> TFISRFAPDQPRKGADILVEALERQGVETVFAYPGGASMEIHQALTRSSSIRNVLPRHEQGGVFAAEGYARSSGKPGICIATSGPGATNLVSGLADALLDSVPLVAITGQVPRRMIGTDAFQETPIVEVTRSITKHNYLVMDVEDIPRIIEEAFFLATSGRPGPVLVDVPKDIQQQLAIPNWEQAMRLPGYMSRMPKPPEDSHLEQIVRLISESKKPVLYVGGGCLNSSDELGRFVELTGIPVASTLMGLGSYPCDDELSLHMLGMHGTVYANYAVEHSDLLLAFGVRFDDRVTGKLEAFASRAKIVHIDIDSAEIGKNKTPHVSVCGDVKLALQGMNKVLENRAEELKLDFGVWRNELNVQKQKFPLSFKTFGEAIPPQYAIKVLDELTDGKAIISTGVGQHQMWAAQFYNYKKPRQWLSSGGLGAMGFGLPAAIGASVANPDAIVVDIDGDGSFIMNVQELATIRVENLPVKVLLLNNQHLGMVMQLEDRFYKANRAHTFLGDPAQEDEIFPNMLLFAAACGIPAARVTKKADLREAIQTMLDTPGPYLLDVICPHQEHVLPMIPSGGTFNDVITEGDGRLEHHHHHH

Acetohydroxyacid synthase (AHAS), also known as acetolactate synthase, is the first enzyme of the branched chain amino acid (BCAA) biosynthesis pathway, and is the target for more than 50 of these commercial herbicides. Since the introduction of these herbicides, 197 site-of-action resistance isolates have been identified. These sites are mainly focused on just eight amino acids 1 with all located in the substrate access channel or the catalytic pocket of AHAS. Here, we show that these mutations can have two effects (i) to reduce binding affinity of the herbicides and (ii) to abolish time-dependent accumulative inhibition, critical to the exceptional effectiveness of this class of herbicide.

Next, the crystal structure of the W574L mutant in complex with CE was determined. When leucine replaces tryptophan, there is a dramatic decrease in the number of enzyme-inhibitor interactions. In the WT complex, the pyrimidine makes π–π interactions and a halogen–π interaction with the indole moiety of W574. In the mutant complex, those interactions are replaced by a hydrophobic interaction between a methyl group of the mutated L574 and the pyrimidine ring of CE. This change is the main factor accounting for the 70-fold loss of affinity of CE for this mutant compared to the WT enzyme. In comparing the structures of the WT and W574L complexes, the most striking difference is a rotation of 38° in the dihedral angle that connects the heterocyclic ring of CE to the sulfonylurea bridge. For the chlorine atom to make an optimal hydrophobic interaction with the side chain of leucine, it is forced towards the region where ThDP is located. Importantly, the position adopted by the chlorine atom in the W574L mutant has the potential to impede accumulative inhibition imposed by CE. The ability of CE to promote accumulative inhibition in the W574L mutant has been virtually abolished relative to WT.> MEHQLLCCEVETIRRAYPDANLLNDRVLRAMLKAEETCAPSVSYFKCVQKEVLPSMRKIVATWMLEVCEEQKCEEEVFPLAMNYLDRFLSLEPVKKSRLQLLGATCMFVASKMKETIPLTAEKLCIYTDNSIRPEELLQMELLLVNKLKWNLAAMTPHDFIEHFLSKMPEAEENKQIIRKHAQTFVALCATDVKFISNPPSMVAAGSVVAAVQGLNLRSPNN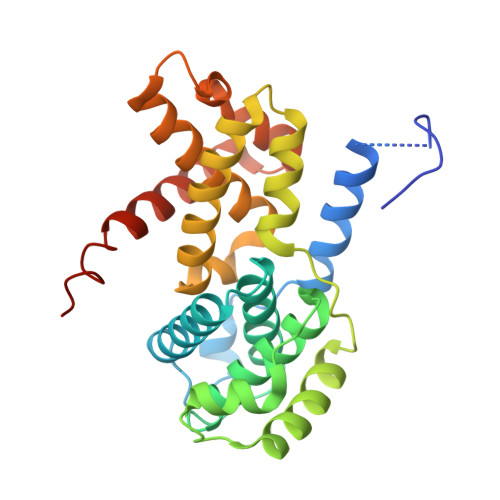FLSYYRLTRFLSRVIKCDPDCLRACQEQIEALLESSLRQAQQNMDPKAA>[2x]GPLGSMSEEQVAQDTEEVFRSYVFYRHQQEQEAEGVAAPADPEMVTLPLQPSSTMGQVGRQLAIIGDDINRRY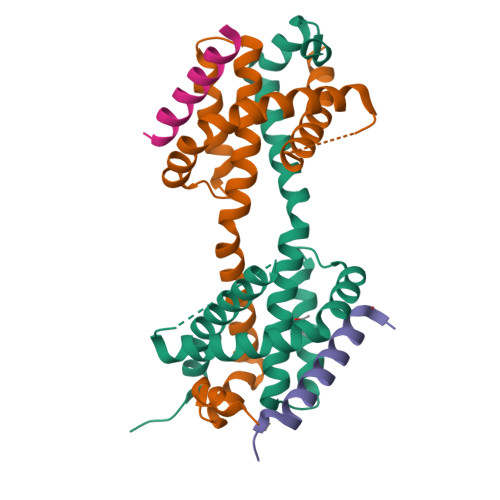DSEFQTMLQHLQPTAENAYEYFTKIATSLFESGINWGRVVALLGFGYRLALHVYQHGLTGFLGQVTRFVVDFMLHHSIARWIAQRGGWVAALNLGNG;>DMRPEIRIAQELRRIGDEFNATYARR[2x]>MGSSHHHHHHSSGRENLYFQGHMEYKKFVEARRELNEKVLSRGTLNTKRFFNLDSAVYRPGKLDVKTKELMGLVASTVLRCDDCIRYH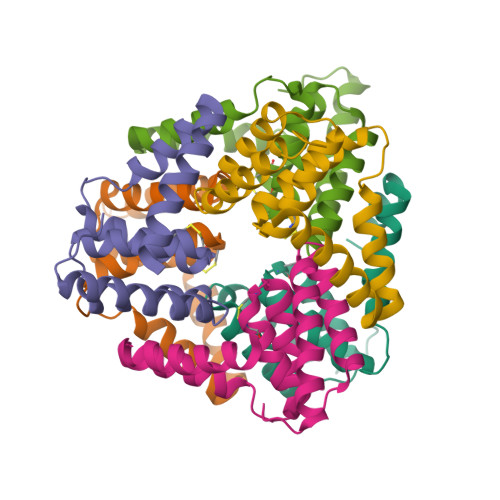LVRCVQEGASDEEIFEALDIALVVGGSIVIPHLRRAVGFLEELREMEKNGETISLGS[6x]>MAERAALEELVKLQGERVRGLKQQKASAELIEEEVAKLLKLKAQLGPDESKQKFVLKTPKGTRDYSPRQMAVREKVFDVIIRCFKRHGAEVIDTPVFELKETLMGKYGEDSKLIYDLKDQGGELLSLRYDLTVPFARYLAMNKLTNIKRYHIAKV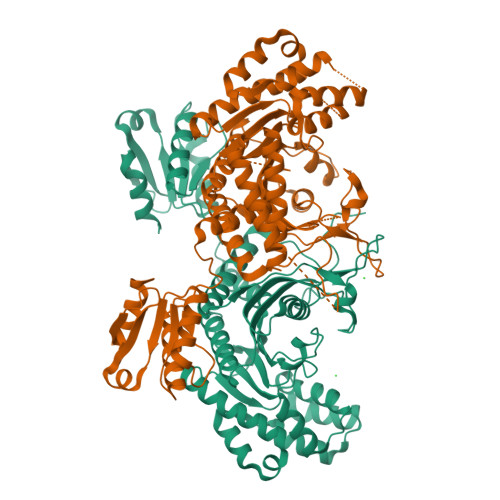YRRDNPAMTRGRYREFYQCDFDIAGNFDPMIPDAECLKIMCEILSSLQIGDFLVKVNDRRILDGMFAICGVSDSKFRTICSSVDKLDKVSWEEVKNEMVGEKGLAPEVADRIGDYVQQHGGVSLVEQLLQDPKLSQNKQALEGLGDLKLLFEYLTLFGIDDKISFDLSLARGLDYYTGVIYEAVLLQTPAQAGEEPLGVGSVAAGGRYDGLVGMFDPKGRKVPCVGLSIGVERIFSIVEQRLEALEEKIRTTETQVLVASAQKKLLEERLKLVSELWDAGIKAELLYKKNPKLLNQLQYCEEAGIPLVAIIGEQELKDGVIKLRSVTSREEVDVRREDLVEEIKRRTGQPLCIC[2x]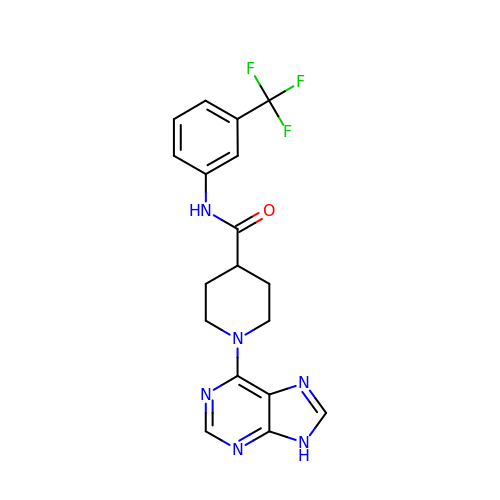1-(9H-purin-6-yl)-N-[3-(trifluoromethyl)phenyl]piperidine-4-carboxamide | C18 H17 F3 N6 O | RSRHDIYCQIWTON-UHFFFAOYSA-N> MNYNNKILVSESGLSQKHLIHGDEELFQHELKTIFARNWLFLTHDSLIPAPGDYVTAKMGIDEVIVSRQNDGSIRAFLNVCRHRGKTLVSVEAGNAKGFVCSYHGWGFGSNGELQSVPFEKDLYGESLNKKCLGLKEVARVESFHGFIYGCFDQEAPPLMDYLGDAAWYLEPMFKHSGGLELVGPPGKVVIKANWKAPAENFVGDAYHVGWTHASSLRSGESIFSSLAGNAALPP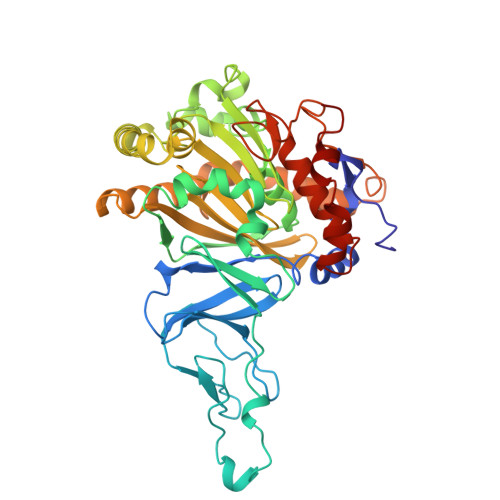EGAGLQMTSKYGSGMGVLWDGYSGVHSADLVPELMAFGGAKQERLNKEIGDVRARIYRSHLNCTVFPNNSMLTCSGVFKVWNPIDANTTEVWTYAIVEKDMPEDLKRRLADSVQRTFGPAGFWESDDNDNMETASQNGKKYQSRDSDLLSNLGFGEDVYGDAVYPGVVGKSAIGETSYRGFYRAYQAHVSSSNWAEFEHASSTWHTELTKTTDR> MSPRVGVTLSGRYRLQRLIATGGMGQVWEAVDNRLGRRVAVKVLKSEFSSDPEFIERFRAEARTTAMLNHPGIASVHDYGESQMNGEGRTAYLVMELVNGEPLNSVLKRTGRLSL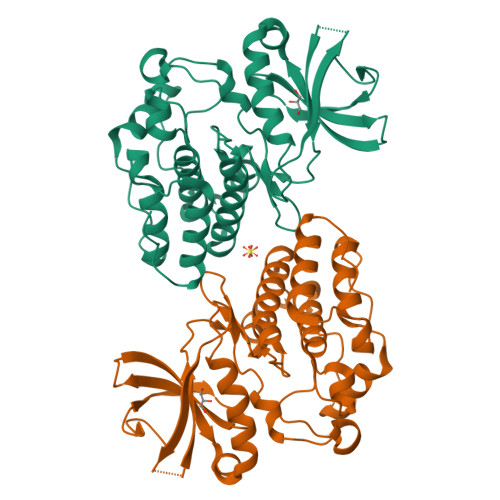RHALDMLEQTGRALQIAHAAGLVHRDVKPGNILITPTGQVKITDFGIAKAVDAAPVTQTGMVMGTAQYIAPEQALGHDASPASDVYSLGVVGYEAVSGKRPFAGDGALTVAMKHIKEPPPPLPPDLPPNVRELIEITLVKNPAMRYRSGGPFADAVAAVRAGRRPPRP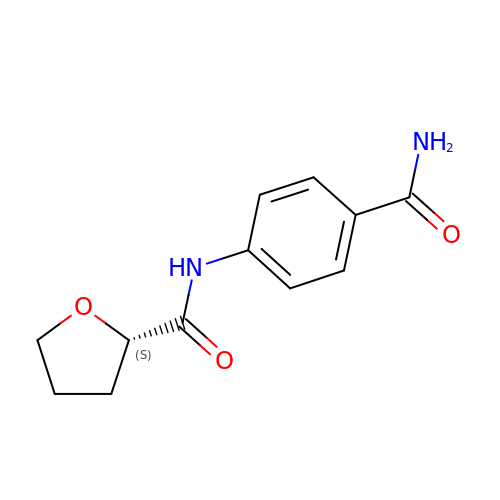(2~{S})-~{N}-(4-aminocarbonylphenyl)oxolane-2-carboxamide | C12 H14 N2 O3 | FSZYBIFIACXSAG-JTQLQIEISA-N> NLYFQSMSIRDLYHARASPFISLEFFPPKTELGTRNLMERMHRMTALDPLFITVTWGAGGTTAEKTLTLASLAQQTLNIPVCMHLTCTNTEKAIIDDALDRCYNAGIRNILALRGDPPIGEDWLDSQSNESPFKYAVDLVRYIKQSYGDKFCVGVAAYPEGHCEGEAEGHEQDPLKDLVYLKEKVEAGADFVITQLFYDVEKFLTFEMLFRERISQDLPLFPGLMPINSYLLFHRAAKLSHASIPPAILSRFPPEIQSDDNAVKSIGVDILIELIQEIYQRTSGRIKGFHFYTLNLEKAIAQIVSQSP

MTHFR catalyzes the physiologically irreversible reduction of 5,10-methylene-tetrahydrofolate (CH2-THF) to 5-methyl-tetrahydrofolate (CH3-THF), a reaction requiring FAD as a cofactor and NADPH as an electron donor. Since the product CH3-THF is exclusively used by methionine synthase, and only the demethylated form (THF) may be recycled back to the folate cycle, MTHFR commits THF-bound one-carbon units to the methionine cycle. Eukaryotic MTHFR orthologs additionally possess a C-terminal regulatory domain that is connected to the catalytic domain by a linker sequence. The MTHFR catalytic domain adopts a TIM-barrel structure evolutionarily conserved across all kingdoms.

In addition to HsMTHFR38–644, we further determined the catalytic domain structure of the yeast homologue MET12 (ScMET121–301) to 1.56 Å resolution. This enables a structural comparison across mammalian (HsMTHFR), low eukaryotic (ScMET12) and bacterial (E. coli, H. influenzae, T. thermophilus) orthologues. Consistent with their sequence conservation, the catalytic domains have highly superimposable folds (main chain RMSD: 1.85 Å), although distinct local differences are found in low homology loop regions and helices. Additionally, the first helix of the catalytic domain (α1) is observed in different orientations among these structures. There is sequence divergence of helix α1 among prokaryotes, lower and higher eukaryotes. In HsMTHFR (which contains, in its biological sequence but not present in the crystallized construct, the serine-rich phosphorylation region N-terminal to the catalytic domain), ScMET12 and T. thermophilus MTHFR, this helix α1 is projected towards the interface between catalytic and regulator domains. In our structures, the FAD ligand adopts a conformation poised to expose the si face of the isoalloxazine ring for the incoming NAPDH and CH2-THF. However, instead of trapping the electron donor or substrate (despite multiple attempts at co-crystallization), the binding site in ScMET121–301 and subunit A of HsMTHFR38–644 is blocked by a crystal packing interaction from a nearby symmetry mate, making π–π stacking interactions with the FAD ligand.> MILDTDYITEDGKPVIRIFKKENGEFKIEYDRTFEPYFYALLKDDSAIEEVKKITAERHGTVVTVKRVEKVQKKFLGRPVEVWKLYFTHPQDVPAI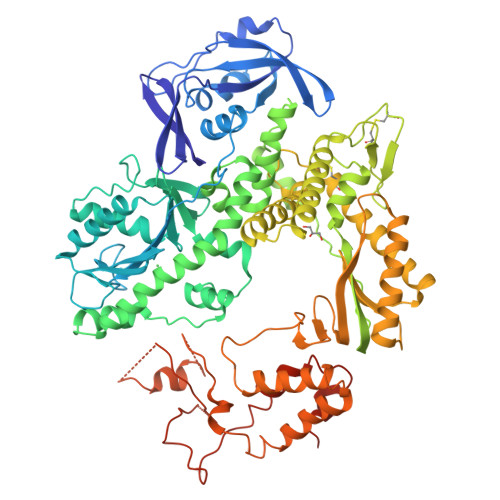RDKIREHPAVIDIYEYDIPFAKRYLIDKGLVPMEGDEELKMLAFDIETLYEEGEEFAEGPILMISYADEEGARVITWKNVDLPYVDVVSTEREMIKRFLRVVKEKDPDVLITYNGDNFDFAYLKKRCEKLGINFALGRDGSEPKIQRMGDRFAVEVKGRIHFDLYPVIRRTINLPTYTLEAVYEAVFGQPKEKVYAEEITTAWETGENLERVARYSMEDAKVTYELGKEFLPMEAQLSRLIGQSLWDVSRSSTGNLVEWFLLRKAYERNELAPNKPDEKELARRRQSYEGGYVKEPERGLWENIVYLDFRSLYPSIIITHNVSPDTLNREGCKEYDVAPQVGHRFCKDFPGFIPSLLGDLLEERQKIKKKMKATIDPIERKLLDYRQRAIKILANSYYGYYGYARARWYCKECAESVTAWGREYITMTIKEIEEKYGFKVIYSDTDGFFATIPGADAETVKKKAMEFLKYINAKLPGALELEYEGFYERGFFVTKKKYAVIDEEGKITTRGLEIVRRDWSEIAKETQARVLEALLKDGDVEKAVRIVKEVTEKLSKYEVPPEKLVIHEQITRDLKDYKATGPHVAVAKRLAARGVKIRPGTVISYIVLKGSGRIGDRAIPFDEFDPTKHKYDAEYYIENQVLPAVERILRAFGYRKEDLRYQKTRQVGLSAWLKPKGT> GSKWKVFIDQINRSLENYEPCSSQNCSCYHGVIEEDLT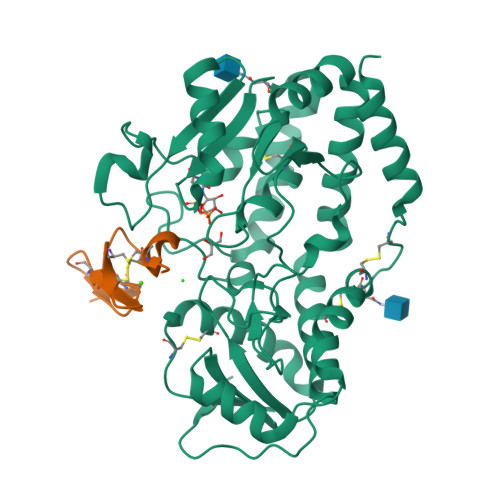PFRGGISRKMMAEVVRRKLGTHYQITKNRLYRENDCMFPSRCSGVEHFILEVIGRLPDMEMVINVRDYPQVPKWMEPAIPVFSFSKTSEYHDIMYPAWTFWEGGPAVWPIYPTGLGRWDLFREDLVRSAAQWPWKKKNSTAYFRGSRTSPERDPLILLSRKNPKLVDAEYTKNQAWKSMKDTLGKPAAKDVHLVDHCKYKYLFNFRGVAASFRFKHLFLCGSLVFHVGDEWLEFFYPQLKPWVHYIPVKTDLSNVQELLQFVKANDDVAQEIAERGSQFIRNHLQMDDITCYWENLLSEYSKFLSYNVTRRKGYDQIIP;> GSDVNECVSNPCQNDATCLDQIGEFQCICMPGYEGVHCEVNT> FMAQILPIRFQEHLQLQNLGINPANIGFSTLTMESDKFICIREKVGEQAQV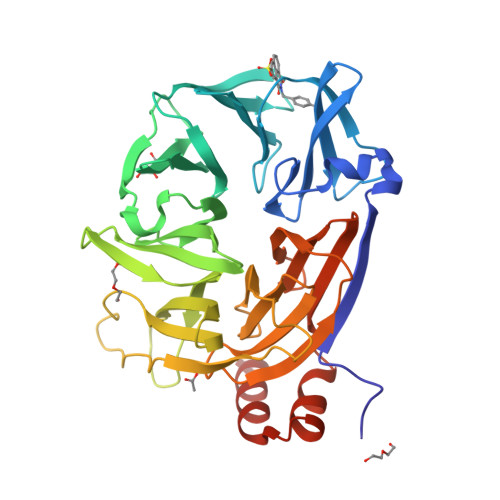VIIDMNDPSNPIRRPISADSAIMNPASKVIALKAGKTLQIFNIEMKSKMKAHTMTDDVTFWKWISLNTVALVTDNAVYHWSMEGESQPVKMFDRHSSLAGCQIINYRTDAKQKWLLLTGISAQQNRVVGAMQLYSVDRKVSQPIEGHAASFAQFKMEGNAEESTLFCFAVRGQAGGKLHIIEVGTPPTGNQPFPKKAVDVFFPPEAQNDFPVAMQISEKHDVVFLITKYGYIHLYDLETGTCIYMNRISGETIFVTAPHEATAGIIGVNRKGQVLSVCVEEENIIPYITNVLQNPDLALRMAVRNNLAGAEELF>[2x]PSVYDAAAQLTADVKKDLRDSWKVIGSDKKGNGVAM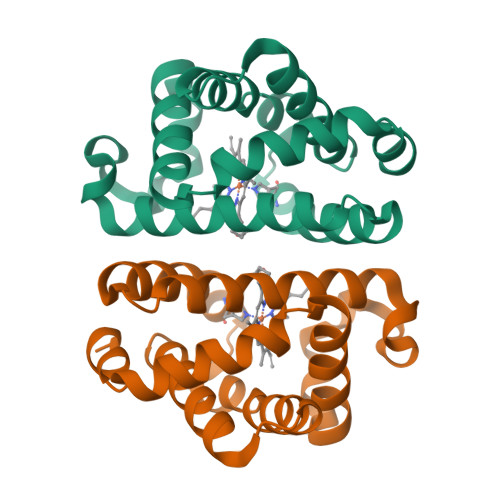MTTLFADNQETIGYFKRLGDVSQGMANDKLRGHSITLMYALQNFIDQLDNPDDLVCVVEKFAVNHITRKISAAEFGKINGPIKKVLASKNFGDKYANAWAKLVAVVQAAL> GPHMKHPLMNVWTLWYLENDRSKSWEDMQNEITSFDTVEDFWSLYNHIKPPSEIKLGSDYSLFKKNIRPMWEDAANKQGGRWVITLNKSSKTDLDNLWLDVLLCLIGEAFDHSDQICGAVINIRGK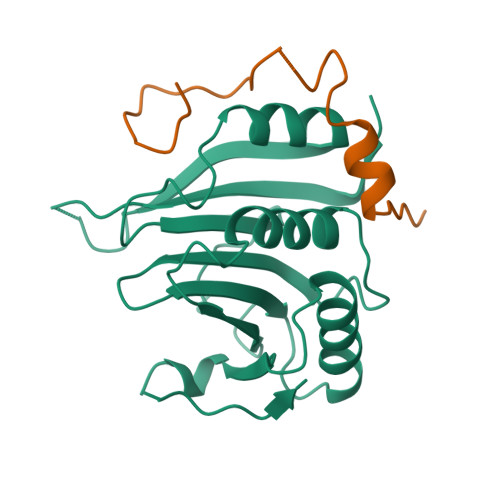SNKISIWTADGNNEEAALEIGHKLRDALRLGRNNSLQYQLHKDTMVKQGSNVKSIYTL;> GPHMRYSKVDLLALRYEGKSRQRPQCSTRLELQTLGFWKI>MAGIKIIKENVDRETFEALAEICPFDAFSYENDKLEVTAACKMCKMCLKKGPEGVLILEEDEKVAIDKSLYRGITVYVDHIEGQIHPVTFELIGKARELAAVIGHPVYALLMGTNITEKADELLKYGVDKVFVYDKPELKHFVIEPYANVLEDFIEKVKPSSILVGATNVGRSLAPRVAARYRTGLTADCTILEMKENTDLVQIRPAFGGNIMAQIVTENTRPQFCTVRYKVFTAPERVNEPWGDVEMMDIEKAKLVSAIEVMEVIKKEKGIDLSEAETIVAVGRGVKCEKDLDMIHEFAEKIGATVACTRPGIEAGWFDARLQIGLSGRTVKPKLIIALGISGAVQFAAGMQNSEYIIAINSDPKAPIFNIAHCGMVGDLYEILPELLTMIEGPENNKDTETISIPEAIETPERM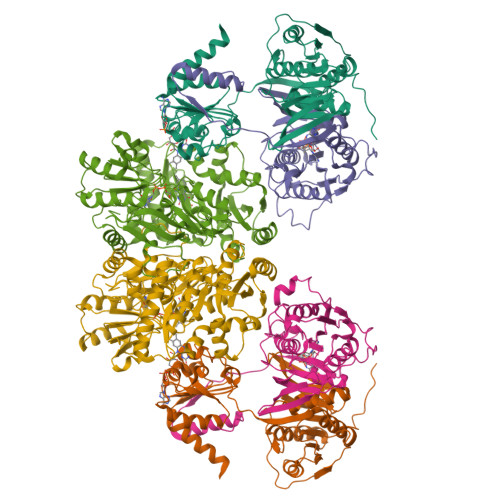VV[2x];>[2x]MSKILVCIKQVPGTSNVEVDPETGVLIRDGVESKLNPYDLFGLETAFRLKEQLGGTITTLSMGPMQSKEVLMESFYMGADEGCLLSDRKFGGADVVATSYTLAQGTKRLGDFDLIICGKQTTDGDTAQVGPEMAEFLGIPHVTNVIKILAADEKGLTLQMNMEESLEIQRVPYPCLITVDKDIYTPRLPSYKRKLDISKNPEIKILTLKDMYDTNEKKYGLSGSPTQVERIFPPESNVEKTSFEGDGKVLAKALLGILTEKKYLG;>[2x]MNYKKVEASDIAAIKELIPAERVFVGTEIGEDFSHDELGSIHSYPEVLIKVTSTEEVSKIMKYAYEHNIPVVVRGSGTGLVGACVPLFGGIMLETTLMNNILELDTENLTVTVEPGVLLMELSKFVEENDLFYPPDPGEKSATIAGNISTNAGGMRAVKYGVTRDYVRGLTVVLANGEIIELGGKIVKNSSGYSLKDLVIGSEGTLCVITKAILKLLPLPKMTLSLLIPFENISDAAGIVPKIIKSKAIPTAIEFMERQTILFAEDFLGKKFPDSSSNAYILLTFDGNTKEQVEAEYETVANLCLAEGAKDVYIVDTVERKDSVWSARGAFLEAIKASTTEMDECDVVVPRNRIAEFIEFTHDLAKEMDVRIPSFGHAGDGNLHIYVCRDELCQADWEAKLAEAMDRMYAKALTFEGLVSGEHGIGYAKRKYLLNDFGTEHLALMAGIKQTFDPKNLLNPKKVCQMA Oligoribonucleases (Orns) are highly conserved DnaQ-fold 3′-5′ exoribonucleases that have been found to carry out the last step of cyclic-di-GMP (c-di-GMP) degradation, that is, pGpG to GMP in several bacteria. Orns are highly conserved DnaQ-fold 3′-5' exoribonucleases with a DEDDh active site motif that degrade short 2- to 5-mer oligoribonucleotides in 3′-5' direction and release monoribonucleotides as reaction products. Removal of pGpG is critical for c-di-GMP homeostasis, as excess uncleaved pGpG can have feedback inhibition on phosphodiesterases, thereby perturbing cellular signaling pathways regulated by c-di-GMP. Removal of pGpG is important to maintain the pool of free nucleotides inside the cell and to prevent mispriming of transcripts and is brought about by Orns.

The structure of Ms_orn in apo form was determined to 1.87 Å resolution to a final Rwork of 17.9% and Rfree of 22.2%. There are four molecules of Ms_orn in one asymmetric unit with two homodimers packed in a side-to-side orientation. The overall structure of Ms_orn consists of the typical RNase-H fold of DnaQ-like exoribonuclease superfamily of proteins consisting of five central β sheets, β5-β4-β1-β2-β3 (arranged in ↑↑↑↓↑ direction) and nine α helices, along with an additional C-terminal helix, α10. Although the terminal residues 197 to 209 of Ms_orn lacked any discernible density, a significant part of the unique C-terminal tail of Ms_orn (residues 181–196) could be built and formed the additional helix, α10, through residues 186 to 195. α10 of one subunit packs against the other subunit of the dimer in a “handshake”-like manner, creating a small flap over the other protomer and is unique to Ms_orn among all bacterial Orn structures. The C-terminal helix hence provides additional interactions for dimer formation by burying an additional ∼1000 Å2 surface area in Ms_orn. The catalytic Asp9, Glu11, Asp110, and Asp162 along with the general base His157, which are characteristic of DEDDh family of exoribonucleases, are conserved in the active site of Ms_orn, as expected. The carboxylate side chains in the active site of Orns usually coordinate two divalent metal ions for substrate binding and catalysis. In the apo form of Ms_orn, we observed only one monovalent cation, K+ ion, that was coordinated by Asp9 and Glu11 in all the chains. The 5' phosphate of modeled pGpG interacts with Ser106 and Ser133 of one subunit and Tyr127 and Arg128 of the other subunit and constricts the active site of Ms_orn. The catalytic pocket of Ms_orn is also lined by Glu11, His63, Val59, and Met12, which prevent accommodation of oligonucleotides that are longer on the 3' end of pGpG, as suggested earlier. The “handshake” conformation of Ms_orn is hence a unique native conformation that aids packing of the dimer and also regulates activity through access of substrates into the active site in both in vivo and in vitro conditions.

>SVRDELVWIDCEMTGLDLKSDRLIEIAVLVTDADLNILGDGLDVVIHADDESLSSMVDVVKQMHARSGLTEEVRRSTVDLATAEEMVLDYIRGHVKQAKTAPLAGNSIATDRGFIARDMPKLDDYLHYRMIDVSSIKELCRRWYPRIYFGQPEKGLAHRALADIHESIRELKYYRATAFVPQPGPSTSDIAAIAAELGPPSSNSADTDSA[4x]>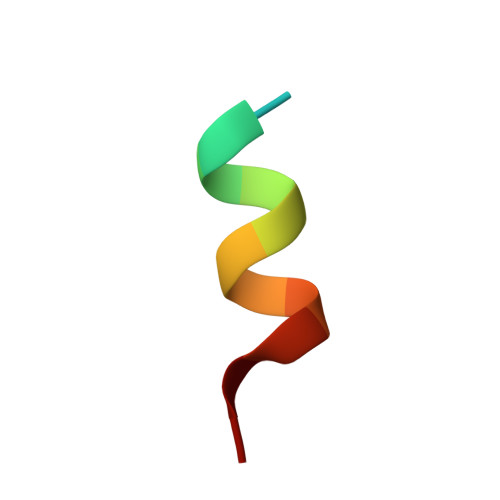 EKHKILHRLLQDS> RPVETPTREIKKLDGLWAFSLDRENCGIDQRWWESALQESRAIAVPGSFNDQFADADIRNYAGNVWYQREVFIPKGWAGQRIVLRFDAVTHYGKVWVNNQEVMEHQGGYTPFEADVTPYVIAGKSVRITVCVNNELNWQTIPPGMVITDENGKKKQSYFHDFFNYAGIHRSVMLYTTPNTWVDDITVVTHVAQDCNHASVDWQVVANGDVSVELRDADQQVVATGQGTSGTLQVVNPHLWQPGEGYLYELCVTAKS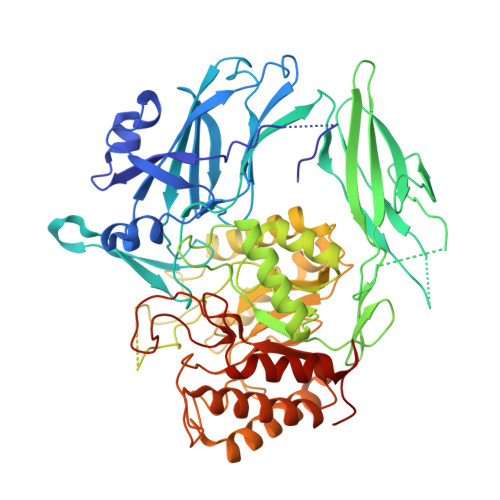QTECDIYPLRVGIRSVAVKGEQFLINHKPFYFTGFGRHEDADLRGKGFDNVLMVHDHALMDWIGANSYRTSHYPYAEEMLDWADEHGIVVIDETAAVGFNLSLGIGFEAGNKPKELYSEEAVNGETQQAHLQAIKELIARDKNHPSVVMWSIANEPDTRPQGAREYFAPLAEATRKLDPTRPITCVNVMFCDAHTDTISDLFDVLCLNRYYGWYVQSGDLETAEKVLEKELLAWQEKLHQPIIITEYGVDTLAGLHSMYTDMWSEEYQCAWLDMYHRVFDRVSAVVGEQVWNFADFATSQGILRVGGNKKGIFTRDRKPKSAAFLLQKRWTGMNFGEKPQQGGKQ>[2x]QSITDYNYKKPLHNDYQILDKSKIFGSNSGSFVMYSMAADAYYIYNEKESRKRYSPNSTYKIYLAMFGLDRHI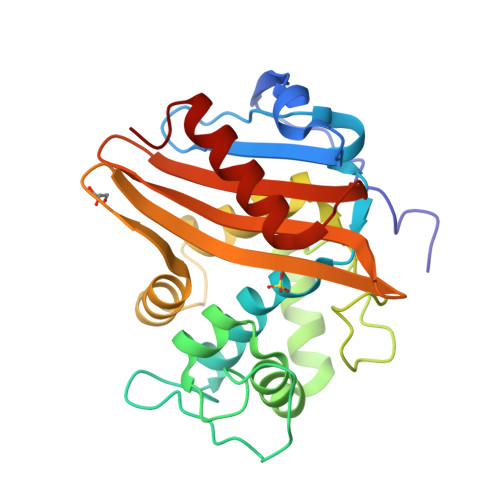INDENSRMSWNHKHYPFDAWNKEQDLNTAMQNSVVWYFERISDQIPKNYTATQLKQLNYGNKNLGSYKSYWMEDSLKISNLEQVIVFKNMMEQNNHFSKKAKNQLSSSLLIKKNEKYELYGKTGTGIVNGKYNNGWFVGYVITNHDKYYFATHLSDGKPSGKNAELISEKILKEMGVLN>[2x]MVHHHHHHNEDICFIAGIGDTNGYGWGIAKELSKRNVKIIFGIWPPVYNIFMKNYKNGKFDNDMIIDKDKKMNILDMLPFDASFDTANDIDEETKNNKRYNMLQNYTIEDVANLIHQKYGKINMLVHSLANAKEVQKDLLNTSRKGYLDALSKSSYS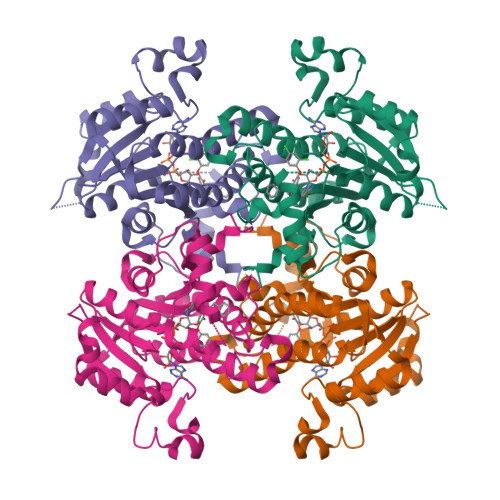LISLCKYFVNIMKPQSSIISLTYHASQKVVPGYGGGMSSAKAALESDTRVLAYHLGRNYNIRINTISAGPLKSRAATAINKLNNTYENNTNQNKNRNSHDVHNIMNNSGEKEEKKNSASQNYTFIDYAIEYSEKYAPLRQKLLSTDIGSVASFLLSRESRAITGQTIYVDNGLNIMFLPDD>[2x]GAMEGFKANLSLLRRPGEKTYTQRCRLFVGNLPADITEDEFKRLFAKYGEPGEVFINKGKGFGFIKLESRALAEIAKAELDDTPMRGRQLRVRFATHAAA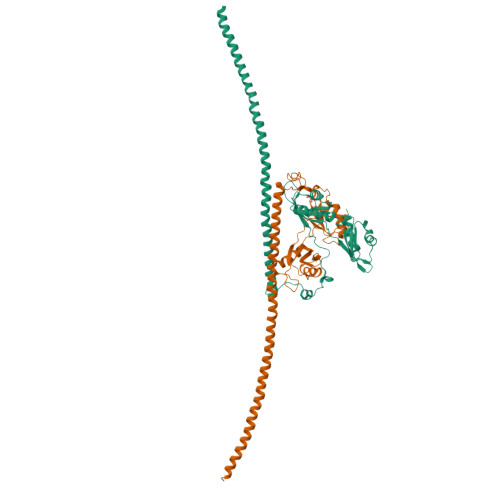LSVRNLSPYVSNELLEEAFSQFGPIERAVVIVDDRGRSTGKGIVEFASKPAARKAFERCSEGVFLLTTTPRPVIVEPLEQLDDEDGLPEKLAQKNPMYQKERETPPRFAQHGTFEYEYSQRWKSLDEMEKQQREQVEKNMKDAKDKLESEMEDAYHEHQANLLRQDLMRRQEELRRMEELHNQEMQKRKEMQLRQEEERRRREEEMMIRQREMEEQMRRQREESYS> MDLSNMESVVESALTGQRTKIVVKVHMPCGKSRAKAMALAASVNGVDSVEITGEDKDRLVVVGRGIDPVRLVALLREKCGLAELLMVELVEKEKTQLAGGKKGAYKKHPTYNLSPFDYVEYPPSAPIMQDINPCSTM;> MAWKDCIIQRY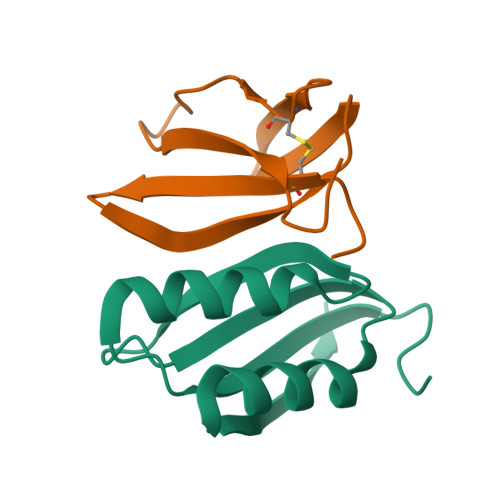KDGDVNNIYTANRNEEITIEEYKVFVNEACHPYPVILPDRSVLSGDFTSAYADDDESCYRHHHHHH> YWPPTRKDRSKRIRLPSGKKCFVFNAKRDQDGELEPVLCFVDS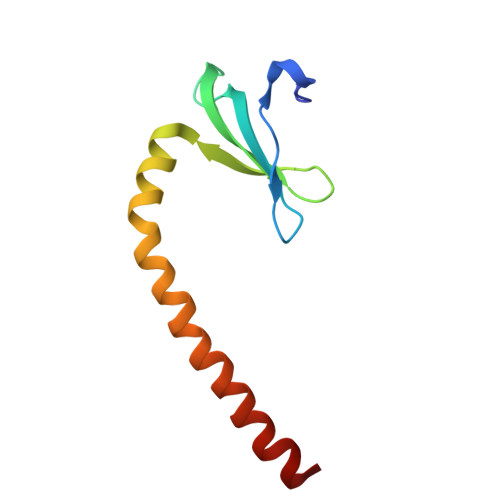QDNLLMWFNEEELLEFEKLMPRLESYYELWEEKASRTRMKEAIVAEAES> GPLGSAKRRKTMQGEGPQLLLSEAVSRAAKAAGARPLTSPESLSRDLEAPEVQESYRQQLRSDIQKRLQE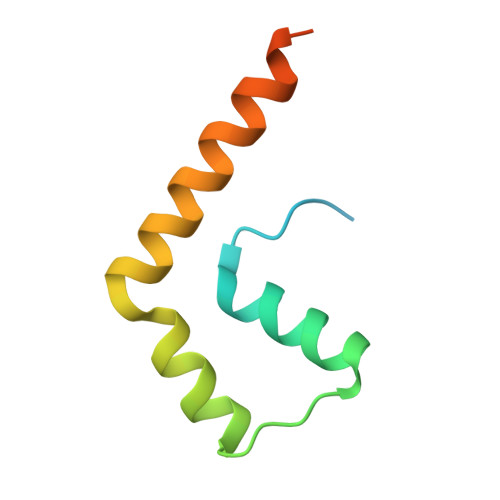DPNYSPQRFPN> MKTATEGRVMRESFLEIIAVVGLSGHDNQGGYNTAGDIKYKTADGVSYDSLWNLFSNVTDEWNKHKSKMVQLMTFPVTNQTEKVPRIGQFGFEKASEFGVPESKRTELSFYQLAYDFEDYDLAFRYTWKFLRDAPSSQIKAYHNQALQADAKLIHRKVMEAIFDNREREADIEGLPYKVYPLYNGDNMIPPEYNGTTFSTGHNHYLVSGGTKIDSADVEMAADHIREHGYTEENGTQLIAFAHKAEIQEVRRFRFGQTNNNSAVANYDFVQSQGESPLYLPNADGLLGKQPQSMWKGLRVKGSYDDVLWIEEPTMPAGYVLFLATGGTLAQQNLVGLR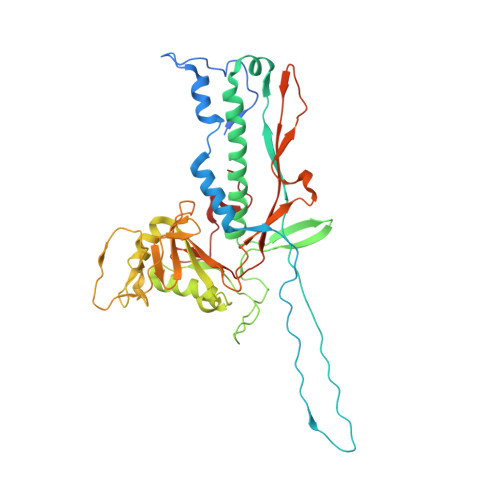EHEDAAWRGLRQIPGNQTRYPLIDSFYQRSFGTGIRQRGGAVVLQIKASGTYDIPTKWTNGGGFE>QKTKQFSVPNLPLNVMSNSRVPSLLNAMVVSPDQAQVVQFQNGRCTLDGQMLGTTTVSASCVARFRGKTFQAPDNRLGINLAEISGEPYHAFESPAPLGFPDFGDGDWHVTATKVTPSQLEANDPVVVGNVQPYNPQFAPHLGTLVVENPTPDQVATGTDLLFNITWLSNRANNRFNPWVIPNYGSTLTEAAQLAPSIFPPGFGETIVYFNSTFPAVGATTHAAIPCLLPQEFVAHFVNEQAPIRGEAALLHYIDPDTHRNLGEFKIYPEGFVTCVPNVGGTGPQSLPTNGVFVFVSWVSRYYQLKPVG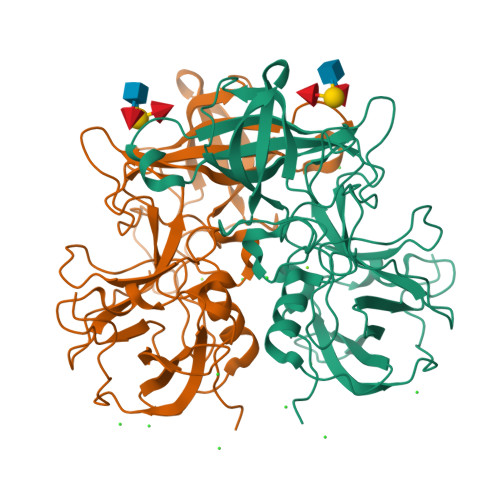TAG[2x]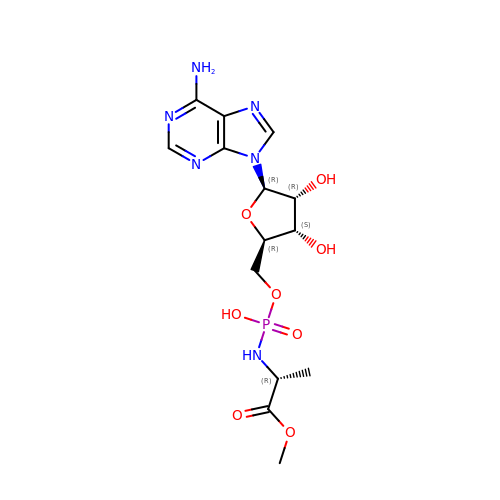[(2~{R},3~{S},4~{R},5~{R})-5-(6-aminopurin-9-yl)-3,4-bis(oxidanyl)oxolan-2-yl]methoxy-~{N}-[(2~{R})-1-methoxy-1-oxidanylidene-propan-2-yl]phosphonamidic acid | C14 H21 N6 O8 P | KHSIAISBDZSYJB-KWGHVAAJSA-N> WGKEGHEIICKIAQTRLDETAAKAVKELLPESAEGDLSSLCLWADRVKFRYHWSSPLHYINTPDACSYQYNRDCKDESGEKGRCV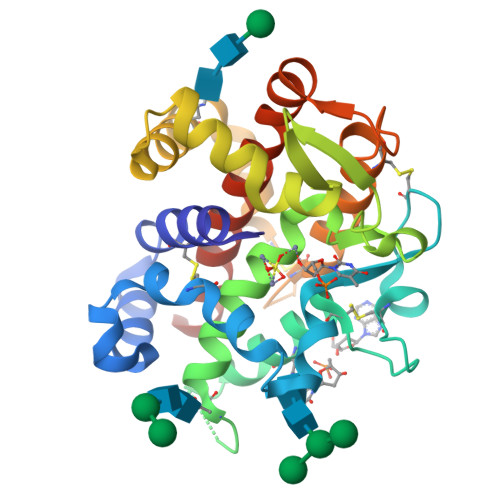AGAIYNYTTQLLSYKTAASSQSEYNLTEALLFVSHFMGDIHQPLHVSYASDKGGNTIEVHWYTRKANLHHIWDSNIIETAEADLYNSALEGMVDALKKNITTEWADQVKRWETCTKKTACPDIYASEGIQAACDWAYKGVTEGDTLEDEYFYSRLPIVYQRLAQGGVRLAATLNRIFGHHHHHH>ASQNSFRIEYDTFGELKVPNDKYYGAQTVRSTMNFKIGGVTERMPTPVIKAFGILKRAAAEVTQDYGLDPKIANAIMKAADEVAEGKLNDHFPLVVWQTGSGTQTNMNVNEVISNRAIEMLGGELGSKIPVHPNDHVNKSQSSNDTFPTAMHIAAAIEVHEVLLPGLQKLHDALDAKSKEFAQIIKIGRTHTQDAVPLTLGQEFSGYVQQVKYAMTRIKAAMPRIYELAAGGTAVGTGLNTRIGFAEKVAAKVAALTGLPFVTAPNKFEALAAHDALVELSGAMNTTACSLMKIANDIRFLGSGPRS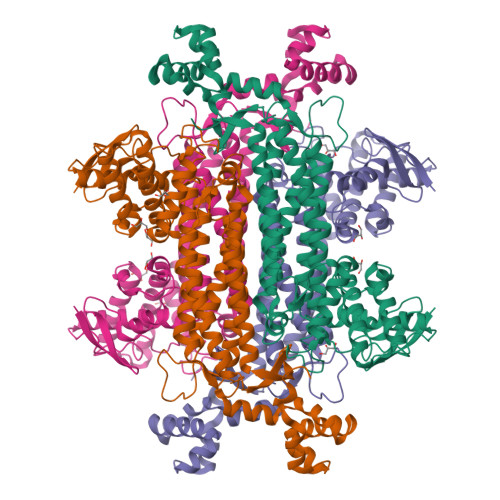GLGELILPENEPGSSIMPGKVNPTQCEAMTMVAAQVMGNHVAVTVGGSNGHFELNVFKPMMIKNVLHSARLLGDASVSFTENCVVGIQANTERINKLMNESLMLVTALNPHIGYDKAAKIAKTAHKNGSTLKETAIELGYLTAEQFDEWVKPKDMLGPK[2x]> MSLSKILIAGCGDLGLELARRLTAQGHEVTGLRRSAQPMPAGVQTLIADVTRPDTLASIVHLRPEILVYCVAASEYSDEHYRLSYVEGLRNTLSALEGAPLQHVFFVSSTGVYG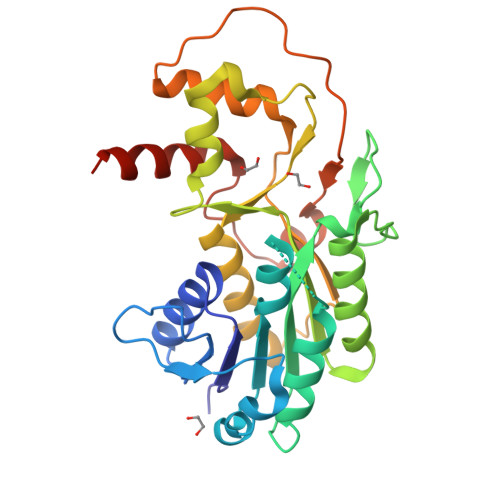QEVEEWLDEDTPPIAKDFSGKRMLEAEALLAAYSSTILRFSGIYGPGRLRMIRQAQTPEQWPARNAWTNRIHRDDGAAFIAYLIQQRSHAVPERLYIVTDNQPLPVHDLLRWLADRQGIAYPAGATPPVQGNKKLSNARLLASGYQLIYPDYVSGYGALLAAMREGHHHHHH> GAMARVTMNEFEYLKLLGKGTFGKVILVKEKATGRYYAMKILKKEVIVAKDEVAHTLTENRVLQNSRHPFLTALKYSFQTHDRLCFVMEYANGGELFFHLSRERVFSEDRARFYGAEIVSALDYLHSEKNVVYRDLKLENLMLDKDGHIKITDFGLCKEGIKDGATMKTFCGTPEYLAPEVLEDNDYGRAVDWWGLGVVMYEMMCGRLPFYNQDHEKLFELILMEEIRFPRTLGPEAKSLLSGLLKKDPKQRLGGGSEDAKEIMQHRFFAGIVWQHVYEKKLSPPFKPQVTSETDTRYFDEEFTAQMITITPPDQD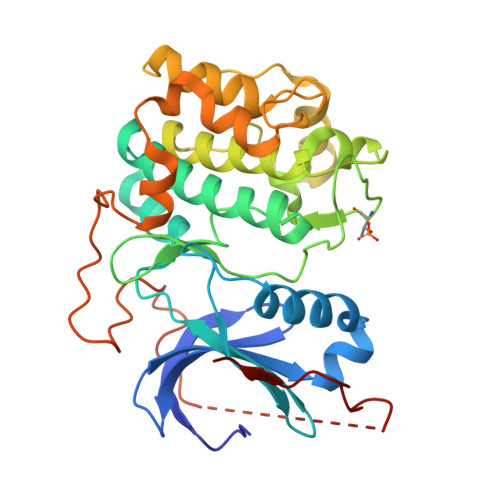DSMECVDSERRPHFPQFDYSASSTA>[2x]MLGLKTSIIGRRVIYFQEITSTNEFAKTSYLEEGTVIVADKQTMGHGALNRKWESPEGGLWLSIVLSPKVPQKDLPKIVFLGAVGVVETLKEFSIDGRIKWPNDVLVNYKAIAGVLVEG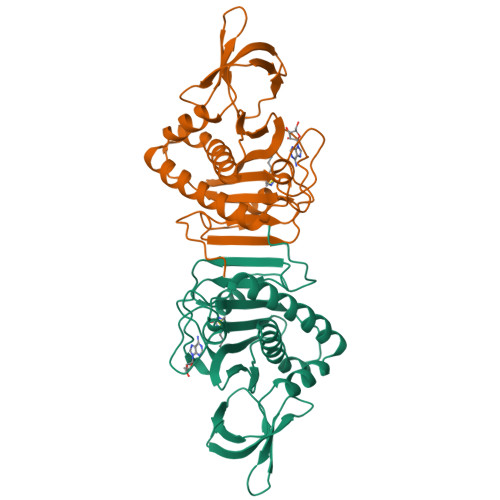KGDKIVLGIGLNVNNKVPNGATSMKLELGSEVPLLSVFRSLITNLDRLYLNFLKNPMDILNLVRDNMILGVRVKILGDGSFEGIAEDIDDFGRLIIRLDSGEVKKVIYGDVSLRFL6-[bis(oxidanyl)methyl]-5~{H}-pyrimidine-2,4-dione | C5 H6 N2 O4 | 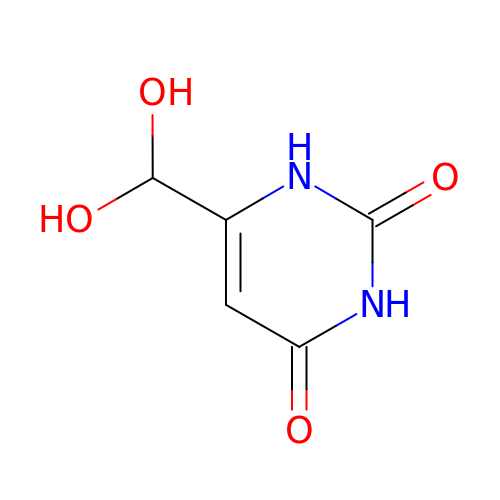DUGHQFVNXIWPEA-UHFFFAOYSA-N> GKDGSPLLCGSIPGLVPKQLRFCRNYIEIMPSVAEGVKLGIQECQHQFRGRRWNCTTIDDSL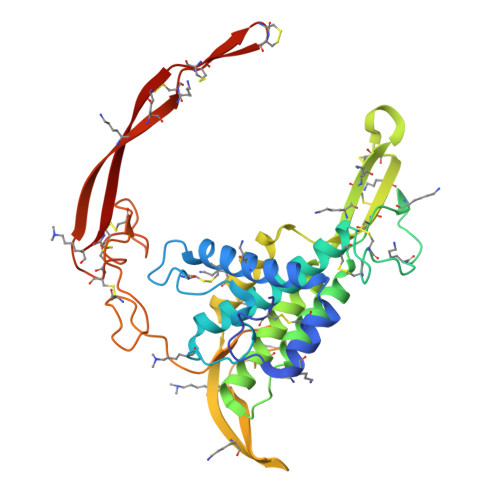AIFGPVLDKATRESAFVHAIASAGVAFAVTRSCAEGTSTICGCDSHHKGPPGEGWKWGGCSEDADFGVLVSREFADARENRPDARSAMNKHNNEAGRTTILDHMHLKCKCHGLSGSCEVKTCWWAQPDFRAIGDFLKDKYDSASEMVVEKHRESRGWVETLRAKYSLFKPPTERDLVYYENSPNFCEPNPETGSFGTRDRTCNVTSHGIDGCDLLCCGRGHNTRTEKRKEKCHCIFHWCCYVSCQECIRIYDVHTCK> MTIHEHDRVSADRGGDSPHTTHALVDRLMAGEPYAVAFGGQGSAWLETLEELVSATGIETELATLVGEAELLLDPVTDELIVVRPIGFEPLQWVRALAAEDPVPSDKHLTSAAVSVPGVLLTQIAATRALARQGMDLVATPPVAMAGHSQGVLAVEALKAGGARDVELFALAQLIGAAGTLVARRRGISVLGDRPPMVSVTNADPERIGRLLDEFAQDVRTVLPPVLSIRNGRRAVVITGTPEQLSRFELYCRQISEKEEADRKNKVRGGDVFSPVFEPVQVEVGFHTPRLSDGIDIVAGWAEKAGLDVALARELADAILIRKVDWVDEITRVHAAGARWILDLGPGDILTRLTAPVIRGLGIGIVPAATRGGQRNLFTVGATPEVARAWSSYAPTVVRLPDGRVKLSTKFTRLTGRSPILLAGMTPTTVDAKIVAAAANAGHWAELAG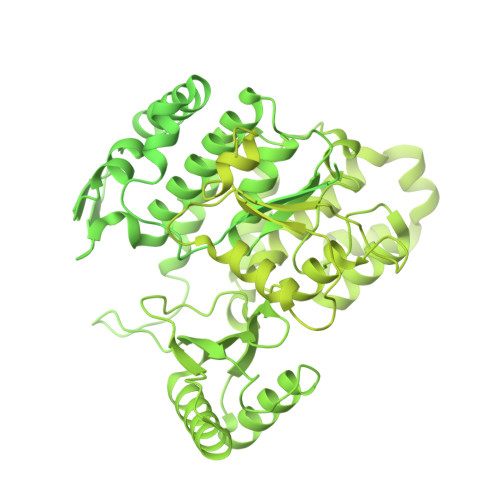GGQVTEEIFGNRIEQMAGLLEPGRTYQFNALFLDPYLWKLQVGGKRLVQKARQSGAAIDGVVISAGIPDLDEAVELIDELGDIGISHVVFKPGTIEQIRSVIRIATEVPTKPVIMHVEGGRAGGHHSWEDLDDLLLATYSELRSRANITVCVGGGIGTPRRAAEYLSGRWAQAYGFPLMPIDGILVGTAAMATKESTTSPSVKRMLVDTQGTDQWISAGKAQGGMASSRSQLGADIHEIDNSASRCGRLLDEVAGDAEAVAERRDEIIAAMAKTAKPYFGDVADMTYLQWLRRYVELAIGEGNSTADTASVGSPWLADTWRDRFEQMLQRAEARLHPQDFGPIQTLFTDAGLLDNPQQAIAALLARYPDAETVQLHPADVPFFVTLCKTLGKPVNFVPVIDQDVRRWWRSDSLWQAHDARYDADAVCIIPGTASVAGITRMDEPVGELLDRFEQAAIDEVLGAGVEPKDVASRRLGRADVAGPLAVVLDAPDVRWAGRTVTNPVHRIADPAEWQVHDGPENPRATHSSTGARLQTHGDDVALSVPVSGTWVDIRFTLPANTVDGGTPVIATEDATSAMRTVLAIAAGVDSPEFLPAVANGTATLTVDWHPERVADHTGVTATFGEPLAPSLTNVPDALVGPCWPAVFAAIGSAVTDTGEPVVEGLLSLVHLDHAARVVGQLPTVPAQLTVTATAANATDTDMGRVVPVSVVVTGADGAVIATLEERFAILGRTGSAELADPARAGGAVSANATDTPRRRRRDVTITAPVDMRPFAVVSGDHNPIHTDRAAALLAGLESPIVHGMWLSAAAQHAVTATDGQARPPARLVGWTARFLGMVRPGDEVDFRVERVGIDQGAEIVDVAARVGSDLVMSASARLAAPKTVYAFPGQGIQHKGMGMEVRARSKAARKVWDTADKFTRDTLGFSVLHVVRDNPTSIIASGVHYHHPDGVLYLTQFTQVAMATVAAAQVAEMREQGAFVEGAIACGHSVGEYTALACVTGIYQLEALLEMVFHRGSKMHDIVPRDELGRSNYRLAAIRPSQIDLDDADVPAFVAGIAESTGEFLEIVNFNLRGSQYAIAGTVRGLEALEAEVERRRELTGGRRSFILVPGIDVPFHSRVLRVGVAEFRRSLDRVMPRDADPDLIIGRYIPNLVPRLFTLDRDFIQEIRDLVPAEPLDEILADYDTWLRERPREMARTVFIELLAWQFASPVRWIETQDLLFIEEAAGGLGVERFVEIGVKSSPTVAGLATNTLKLPEYAHSTVEVLNAERDAAVLFATDTDPEPEPEEDEPVAESPAPDVVSEAAPVAPAASSAGPRPDDLVFDAADATLALIALSAKMRIDQIEELDSIESITDGASSRRNQLLVDLGSELNLGAIDGAAESDLAGLRSQVTKLARTYKPYGPVLSDAINDQLRTVLGPSGKRPGAIAERVKKTWELGEGWAKHVTVEVALGTREGSSVRGGAMGHLHEGALADAASVDKVIDAAVASVAARQGVSVALPSAGSGGGATIDAAALSEFTDQITGREGVLASAARLVLGQLGLDDPVNALPAAPDSELIDLVTAELGADWPRLVAPVFDPKKAVVFDDRWASAREDLVKLWLTDEGDIDADWPRLAERFEGAGHVVATQATWWQGKSLAAGRQIHASLYGRIAAGAENPEPGRYGGEVAVVTGASKGSIAASVVARLLDGGATVIATTSKLDEERLAFYRTLYRDHARYGAALWLVAANMASYSDVDALVEWIGTEQTESLGPQSIHIKDAQTPTLLFPFAAPRVVGDLSEAGSRAEMEMKVLLWAVQRLIGGLSTIGAERDIASRLHVVLPGSPNRGMFGGDGAYGEAKSALDAVVSRWHAESSWAARVSLAHALIGWTRGTGLMGHNDAIVAAVEEAGVTTYSTDEMAALLLDLCDAESKVAAARSPIKADLTGGLAEANLDMAELAAKAREQMSAAAAVDEDAEAPGAIAALPSPPRGFTPAPPPQWDDLDVDPADLVVIVGGAEIGPYGSSRTRFEMEVENELSAAGVLELAWTTGLIRWEDDPQPGWYDTESGEMVDESELVQRYHDAVVQRVGIREFVDDGAIDPDHASPLLVSVFLEKDFAFVVSSEADARAFVEFDPEHTVIRPVPDSTDWQVIRKAGTEIRVPRKTKLSRVVGGQIPTGFDPTVWGISADMAGSIDRLAVWNMVATVDAFLSSGFSPAEVMRYVHPSLVANTQGTGMGGGTSMQTMYHGNLLGRNKPNDIFQEVLPNIIAAHVVQSYVGSYGAMIHPVAACATAAVSVEEGVDKIRLGKAQLVVAGGLDDLTLEGIIGFGDMAATADTSMMCGRGIHDSKFSRPNDRRRLGFVEAQGGGTILLARGDLALRMGLPVLAVVAFAQSFGDGVHTSIPAPGLGALGAGRGGKDSPLARALAKLGVAADDVAVISKHDTSTLANDPNETELHERLADALGRSEGAPLFVVSQKSLTGHAKGGAAVFQMMGLCQILRDGVIPPNRSLDCVDDELAGSAHFVWVRDTLRLGGKFPLKAGMLTSLGFGHVSGLVALVHPQAFIASLDPAQRADYQRRADARLLAGQRRLASAIAGGAPMYQRPGDRRFDHHAPERPQEASMLLNPAARLGDGEAYIG> MGSSHHHHHHMTCTLRDLNSLLEISSVRNDAQCCRCPAHNPSTAFAPTTKVRVSSDVRGIFALPVQKDHKPYNGLSPEHLETMKAVSLMLDAAGPKLEDGISKAKELLEERINPELMRDALGIYLTHSKDAQQRKIFPPPLKNHPFFSTKTRRPANVAGEICTADTLHGHALLSYWRDDYDLNDSHYYWHMVYRGAGGDNSKNVGDFDRHGEVFLYVHSQMVARYETESLCWSLPLVRPWNQYDDFLENGYAPISSLIEHYGGYPPFSTWYSIRNPDMPDTLNVTIPRARLEEWRDNIYAAIRKGQFETTSKDKPLVLTRDNCLNFVGGILDAQYPSLNKLLGGCSLDEERYGNLHNYGLGKFAEMAYRNKPGEKSPYGLTISNFGAPRDPCFWRWYKHLQYYGRLAATRYPQDITAHRAEVVLSNLVVRLQDRSSPHYLDGHITTFL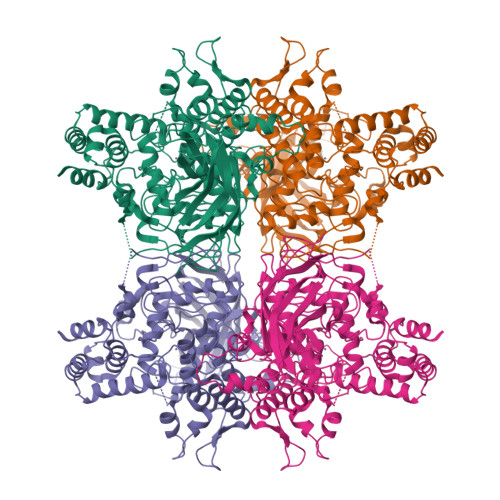GPPAVNFMESKAKLGHEPYEWNVQVKSCRRSPPSKENPQTLTLRLFIAAEDLMNDYHSWIEMDRATVQLTDESAITKVRLDTDSSVARKMGNYGEPDPRYASAVFRHGWPQNLMLPVGKVEGMPFVAFCIATDDGIPDPAPAPPFHHYHDPRGMGYPFNRAWTQLTEDSTGKASIRTIISNAELYPFITSTTFKIYRTTKFETKQIIQPTTVTWFNTIRGYFKDADRACMRSEYGYDLYNYDHVMLHADAILDATASKRMPLQMGKYTQDNPDPEHPLWTVKMCENFRAWLLNGCPKGTDP ACETYLTHIOCHOLINE | C7 H16 N O S | 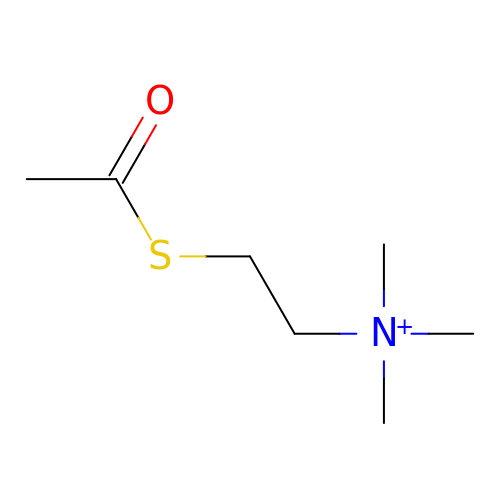GFFIJCYHQYHUHB-UHFFFAOYSA-N> GLPTTTLPGSGQFLTTDDRQSPSALPSYEPTPRIHIPGKVRNLLEIIQVGTLIPMNNTGTNDNVTNYLIPLHADRQNEQIFGTKLYIGDGVFKTTLLGEIAQYYTHWSGSLRISLMYTGPALSSA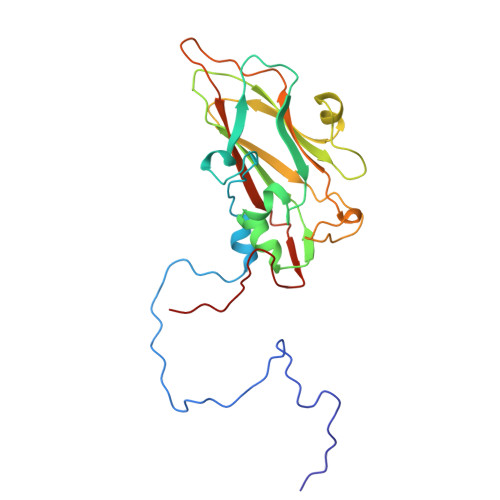KIILAYTPPGTRGPEDKKEAMLGTHVVWDIGLQSTIVMTIPWTSGVQFRYTDPDTYTSAGYLSCWYLTSLILPPQTSGQVYLLSFISACPDFKLRLMKDTQTISQTDALTE> MSQYSENIIIGAGAAGLFCAAQLAKLGKSVTVFDNGKKIGRKILMSGGGFCNFTNLEVTPAHYLSQNPHFVKSALARYTNWDFISLVAEQGITYHEKELGQLFCDEGAEQIVEMLKSECDKYGAKILLRSEVSQVERIQNDEKVRFVLQVNSTQWQCKNLIVATGGLSMPGLGATPFGYQIAEQFGIPVIPPRASLVPFTYRETDKFLTALSGI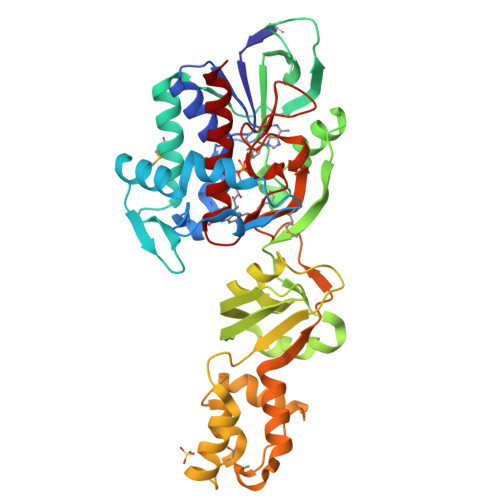SLPVTITALCGKSFYNQLLFTHRGISGPAVLQISNYWQPTESVEIDLLPNHNVEEEINQAKQSSPKQMLKTILVRLLPKKLVELWIEQGIVQDEVIANISKVRVKNLVDFIHHWEFTPNGTEGYRTAEVTMGGVDTKVISSKTMESNQVSGLYFIGEVLDVTGWLGGYNFQWAWSSAYACALSISRQ>MPGIMKNKKLLCSVCFLFAFMSALWGQNITVKGNVTSKTDGQPIIGASVVETTATTNGTITDFDGNFTLSVPVNSTLKITYIGYKPVTVKAAAIVNVLLEEDTQMVDEVVVTGYTTQRKADLTGAVSVVKVDEIQKQGENNPVKALQGRVPGMNITADGNPSGSATVRIRGIGTLNNNDPLYIIDGVPTKAGMHELNGNDIESIQVLKDAASASIYGSRAANGVIIITTKQGKKGQIKINFDASVSASMYQSKMNVLNTEQYGRAMWQAYVNDGENPNGNALGYAYNWGYNADGNPVLYGMTLSKYLDSKNTMPVADTDWFDEITRTGVIQQYNLSVSNGSEKGSSFFSLGYYKNLGVIKDTDFDRFSARMNSDYKLIDDILTIGQHFTLNRTSEVQAPGGIIETALDIPSAIPVYASDGSWGGPVGGWPDRRNPRAVLEYNKDNRYTYWRMFGDAYVNLTPFKGFNLRSTFGLDYANKQARYFTYPYQEGTQTNNGKSAVEAKQEHWTKWMWNAIATYQLEVGKHRGDVMIGMELNREDDSHFSGYKEDFSILTPDYMWPDAGSGTAQAYGAGEGYSLVSFFGKMNYSYADRYLLSLTLRRDGSSRFGKNHRYATFPSVSLGWRITQENFMKELTWLDDLKLRASWGQTGNQEISNLARYTIYAPNYGTTDSFGGQSYGTAYDITGSNGGGVLPSGFKRNQIGNDNIKWETTTQTNVGIDFSLFKQSLYGSLEYYYKKATDILTEMAGVGVLGEGGSRWINSGAMKNQGFEFNLGYRNKTAFGLTYDLNGNISTYRNEILELPETVAANGKFGGNGVKSVVGHTYGAQVGYIADGIFKSQDEVDNHATQEGAAVGRIRYRDIDHNGVIDERDQNWIYDPTPSFSYGLNIYLEYKNFDLTMFWQGVQGVDIISDVKKKSDFWSASNVGFLNKGTRLLNAWSPTNPNSDIPALTRSDTNNEQRVSTYFVENGSFLKLRNIQLGYTVPAVISKKMRMDRLRFYCSAQNLLTIKSKNFTGEDPENPNFSYPIPVNITFGLNIGF[2x];>MKKIIYIATIGITLLTTSCDDFLDRQVPQGIVTGDQIASPEYVDNLVISAYAIWATGDDINSSFSLWNYDVRSDDCYKGGSGTEDGGVFNALEISKGINTTDWNINDIWKRLYQCITRANTALQSLDQMDEKTYPLKNQRIAEMRFLRGHAHFMLKQLFKKIVIVNDENMEPDAYNELSNTTYTNDEQWQKIADDFQFAYDNLPEVQIEKGRPAQAAAAAYLAKTYLYKAYRQDGADNALTGINEEDLKQVVKYTDPLIMAKGGYGLETDYSMNFLPQYENGAESVWAIQYSINDGTYNGNLNWGMGLTTPQILGCCDFHKPSQNLVNAFKTDSQGKPLFSTYDNENYEVATDNVDPRLFHTVGMPGFPYKYNEGYIIQKNDDWSRSKGLYGYYVSLKENVDPDCDCLKKGSYWASSLNHIVIRYADVLLMRAEALIQLNDGRITDAISLINEVRSRAAGSTMLIFNYKEDYGVNFKVTPYDLKAYAQDEAMKMLKWERRVEFGMESSRFFDLVRWGEAKDVINAYYVTEASRCSIYKNAGFTENKNEYLPVPFEQISASNGNYTQNFGWAAAAHHHHHH[2x]

Glycan uptake across the bacterial outer membrane (OM) of these bacteria is mediated by SusCD protein complexes, comprising a membrane-embedded barrel and a lipoprotein lid, that is thought to open and close to facilitate substrate binding and transport. Here we show that for both the levan and dextran utilisation systems of Bacteroides thetaiotaomicron, the additional OM components assemble on the core SusCD transporter, forming stable glycan utilising machines which we term ‘utilisomes’. Transport-competent FOS are generated from levan by a surface-exposed lipoprotein, a GH32-family levan endo-glycanase (GHlev), while an SGBP (SGBPlev) is thought to recruit levan at the cell surface. Single particle cryogenic electron microscopy (cryoEM) structures in the absence and presence of substrate reveal concerted conformational changes that demonstrate the mechanism of substrate capture, and rationalise the role of each component in the utilisome.

All SusDlev lids are closed, tightly capping the extracellular face of the SusClev barrels, relative to the open position in the apo utilisomes. 3D classification reveals that the major source of heterogeneity present in the data was the presence of sub-complexes missing one or more accessory lipoproteins (ED Fig. 3b), so to probe substrate binding within the closed transporter complex, we first performed targeted refinement of the SusCDlev core, using particle subtraction to remove the signal for GHlev and SGBPlev from the images. FOS1 is found at the interface between SusClev and SusDlev, and consists of six β2,6-linked fructose units with a β2,1 decoration on fructose-4 (numbered from the non-reducing end). A second binding site (FOS2) most likely consists of four β2,6-linked fructose units, and is bound at the bottom of the SusClev cavity where it contacts the top of the plug domain. In the apo structure, this region (SusClev loop 8) is mostly unresolved, likely as an artefact of masking during image processing, whereas in the substrate-bound complex SusClev loop 8 contacts SusDlev and FOS1 via F649. In the substrate-bound structure, W685, which sits at the base of loop 8, shifts inwards, nudging F583 up and S193 down. This in turn results in a downward shift of a plug loop containing S193. In the apo structure, Y191, which is part of the same plug loop, forms a triple aromatic stack with Y89 and F558 that links the wall of the barrel (F558), the TonB box (Y89) and the plug domain (Y191). When the plug loop with Y191 shifts towards the periplasm, this stacking interaction is broken, resulting in release of the N-terminus and an ~35 Å shift of R93, which in the substrate-bound complex is the first visible residue. This would plausibly make the TonB box (D82-G88) available for interaction with TonB to disrupt the plug and generate a channel for substrate diffusion into the periplasmic space (Supplementary Discussion).>MHHHHHHMNFNVSLMEKLKWKIKCIENKFLNYRLTTNETVVAETEYGKVKGVKRLTVYDDSYYSFEGIPYAQPPVGELRFKAPQRPTPWAGVRDCCNHKDKSVQVDFITGKVCGSEDCLYLSVYTNNLNPETKRPVLVYIHGGGFIIGENHRDMYGPDYFIKKDVVLINIQYRLGALGFLSLNSEDLNVPGNAGLKDQVMALRWIKNNCANFGGNPDNITVFGESAGAASTHYMMLTEQTRGLFHRGILMSGNAICPWANTQCQHRAFTLAKLAGYKGEDNDKDVL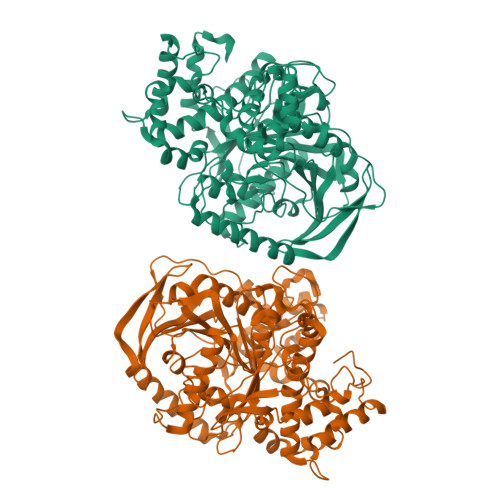EFLMKAKPQDLIKLEEKVLTLEERTNKVMFPFGPTVEPYQTADCVLPKHPREMVKTAWGNSIPTMMGNTSYEGLFFTSILKQMPLLVKELETCVNFVPSELADAERTAPETLEMGAKIKKAHVTGETPTADNFMDLCSHFYFWFPMHRLLQLRFNHTSGTPVYLYRFDFDSEDLINPYRIMRSGRGVKGVSHTDELTYFFWNQLAKRMPKESREYKTIERMTGIWTQFATTGNPYSNEIEGMENVSWDPIEKSDEVYKCLNISDELKMIDVPEMGKIKQWESMFEKHRDLF[2x]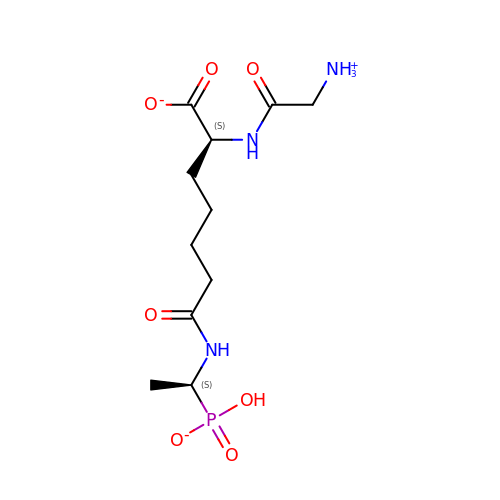GLYCYL-L-A-AMINOPIMELYL-E-(D-2-AMINOETHYL)PHOSPHONATE | C11 H21 N3 O7 P | DREJXTKPUGMERN-YUMQZZPRSA-M> SEVSDTNLYSPFKPRNYQLELALPAMKGKNTIICAPTGCGKTFVSLLICEHHLKKFPQGQKGKVVFFANQIPVYEQNKSVFSKYFERHGYRVTGISGATAENVPVEQIVENNDIIILTPQILVNNLKKGTIPSLSIFTLMIFDECHNTSKQHPYNMIMFNYLDQKLGGSSGPLPQVIGLTASVGVGDAKTTDEALDYICKLCASLDASVIATVKHNLEELEQVVYKPQKFFRKVESRISDKFKYIIAQLMRDTESLAKRICKDLENLSQIQNREFGTQKYEQWIVTVQKACMVFQMPDKDEESRICKALFLYTSHLRKYNDALIISEHARMKDALDYLKDFFSNVRAAGFDEIEQDLTQRFEEKLQELESVSRDPSNENPKLEDLCFILQEEYHLNPETITILFVKTRALVDALKNWIEGNPKLSFLKPGILTGRGKTNQNTFFGMTLPAQKCILDAFKASGDHNILIATSVADEGIDIAQCNLVILYEYVGNVIKMIQTRGRGRARGSKCFLLTSNAGVIEKEQINMYKEKMMNDSILRLQTWDEAVFREKILHIQTHEKFIRDSQEKPKPVPDKENKKLLCRKCKALACYTADVRVIEDCHYTVLGDAFKECFVSRPHPKPKQFSSFEKRAKIFCARQNCSHDWGIHVKYKTFEIPV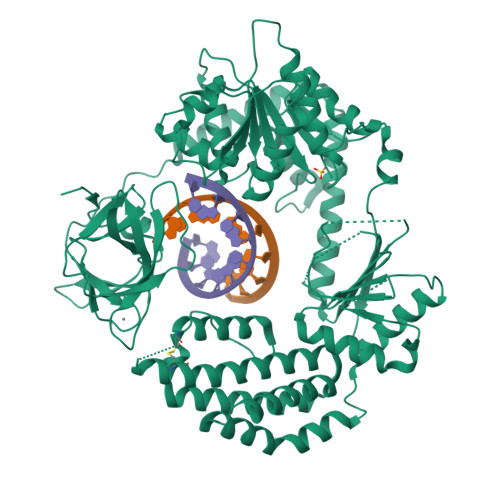IKIESFVVEDIATGVQTLYSKWKDFHFEKIPFDPAEMSK>AVIPRGAVPVASDLSLVSILSSAANDSSIESEARSIASLIASEIVSKIGKTEFSRSTKDAKSVQEAFDKIQSIFADGTPDFLKMTREILTVGLIPADILSFLNGYLNLDLNSIHNRNPSPKGQAIYPVKAPGDARYSVAENALRAAIHIP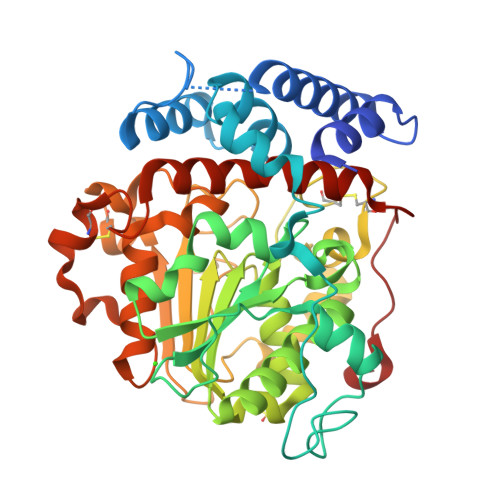ASFGYGKNGKKPVILVPGTATPAGTTYYFNFGKLGSAADADVVWLNIPQASLNDVQINSEYVAYAINYISAISESNVAVLSWSQGGLDTQWALKYWPSTRKVVDDFIAISPDFHGTVMRSLVCPWLAALACTPSLWQQGWNTEFIRTLRGGGGDSAYVPTTTIYSTFDEIVQPMSGSQASAILSDSRAVGVSNNHLQTICGGKPAGGVYTHEGVLYNPLAWALAVDALSHDGPGDPSRLDLDVVCGRVLPPQLGLDDLLGTEGLLLIALAEVLAYKPKTFGEPAIASYAH[3x]>[3x]MSINSREVLAEKVKNAVNNQPVTDMHTHLFSPNFGEILLWDIDELLTYHYLVAEVMRWTDVSIEAFWAMSKREQADLIWEELFIKRSPV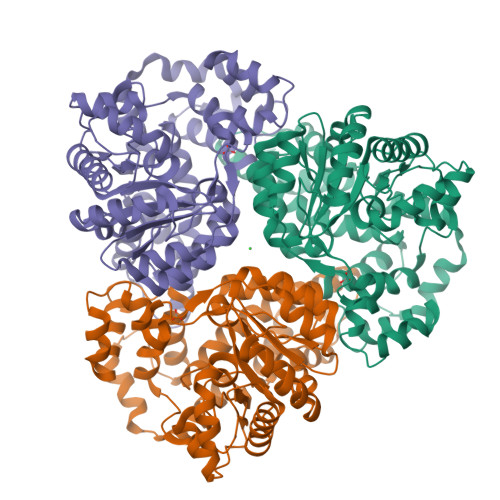SEACRGVLTCLQGLGLDPATRDLQVYREYFAKKTSEEQVDTVLQLANVSDVVMTNDPFDDNERISWLEGKQPDSRFHAALRLDPLLNEYEQTKHRLRDWGYKVNDEWNEGSIQEVKRFLTDWIERMDPVYMAVSLPPTFSFPEESNRGRIIRDCLLPVAEKHNIPFAMMIGVKKRVHPALGDAGDFVGKASMDGVEHLLREYPNNKFLVTMLSRENQHELVVLARKFSNLMIFGCWWFMNNPEIINEMTRMRMEMLGTSFIPQHSDARVLEQLIYKWHHSKSIIAEVLIDKYDDILQAGWEVTEEEIKRDVADLFSRNFWRFVGRNDHVTSVKVEQQT> TGRPEWIWLALGTALMGLGTLYFLVKGMGVSDPDAKKFYAITTLVPAIAFTMYLSMLLGYGLTMVPFGGEQNPIYWARYADWLFTTPLLLLDLALLVDADQGTILALVGADGIMIGTGLVGALTKVYSYRFVWWAISTAAMLYILYVLFFGFTSKAESMRPEVASTFKVLRNVTVVLWSAYPVVWLIGSEGAGIVPLNIETLLFMVLDVSAKVGFGLILLRSRAIFGEAE

In the case of bR, the retinal chromophore forms a Schiff-base (SB) linkage with a lysine residue at position 216 (Lys216). Retinal takes an all-trans conformation in the light-adapted resting state. The light absorption causes the isomerization of a double bond at C13−C14 of retinal from a trans to cis conformation. In the reaction cycle of bR, a single proton is transported from the inside to the outside of the plasma membrane.

Diffraction data from a crystal including the K intermediate at ~1.3 Å were collected at 15 K with an absorbed dose of 0.05 MGy. Subsequently, diffraction data of the ground state were collected from the same crystal after irradiation of red light. The average I/σ(I) value for the highest shell (1.42–1.33 Å) was a sufficiently high value of ~1.4, when the resolution limit was determined as a shell with CC1/2 of ~0.5. As for the ground state, X-ray diffraction data from crystal I and II were measured after the activation with green laser and subsequent restoration with red laser, whereas data from crystal III were measured before the activation. Nevertheless, three structures are also nearly identical as in the case of the K structures. This implies that the process of activation does not affect the ground state structure. On the other hand, the distance between Asp212 and W402 is shortened to 3.08 Å, although the distance in the ground state is 3.40 Å. Although the distance between Nζ of Lys216 and Oδ1 of Asp212 in the ground state is 3.93 Å, indicating no significant interaction, it decreases to 3.27 Å in the K intermediate. Asp115 forms two hydrogen bonds with Thr90, both in the ground state and the K intermediate.>MGTFTLHQGQTNLIKSFFRNYYLNAELELPKDMELREFALQPFGSDTYVRHLSFSSSEELRDYLVNRNLPLHLFYSSARYQLPSARNMEEKAWMGSDLLFDIDADHLCKLRSIRFCPVCGNAVVSEKCERDNVETLEYVEMTSECIKRGLEQTRNLVEILEDDFGLKPKVYFSGNRGFHVQVDCYGNCALLDSDERKEIAEYVMGIGVPGYPGGSENAPGWVGRKNRGINGVTIDEQVTIDVKRLIRIPNSLHGKSGLIVKRVPNLDDFEFNETLSPFTGYTIFLPYITIETEVLGSIIKLNRGIPIKIKSSIGIYLHLRNLGEVKAYVR[2x];>MALDVKKYPFIKSLDDELKKYGGGITLTDLLLNSTTLIDQAKDRIQKTKSGDELPHYVSYNEPVLVFYTTLLSLAILNDVKLIRRYAYAEAKQFRSLLHTENEENLLEISKLLDLKINRCDPIKFYLEKKRRIIQKEFCVHFIDYLKYTKDLKEDWKLSGQILHKGYVYLDKNQLIGLIAESIKSKIVEMIRPLNLKEIPEKLKSLIERRGIIPPCIENILAKEKLNEEEIRTLITFYIDIGKGLSGIVSIMKKYNVSNVEDLYRKYRGDKGTRYIVYSCAKMKQLGLCVSSCNVKNPLQLYFLSNE[2x];>[2x]MSQEKKAKKIILHYPDDTPAGYIEYAEGSSSIYDNEGNFLFKVEGKFPPQPKKSSDYSWIEKVLEMGLQDSRKRFILYVASRYLVNVKGVNEDEALQTLKEFYYKLQSGKVYESWLKSVINGVKKKGLLPWSLKRIEERDKEMYNEIIRVLKNS

Initiation of DNA synthesis during DNA replication relies on a specialised DNA-dependent RNA polymerase, known as primase. In archaea and eukarya, primase is a constitutive heterodimer of a catalytic subunit, PriS or Pri1, and a regulatory subunit, PriL or Pri27. PriX is required for primase activity and the protein is encoded by a gene that is essential for viability. We have shown that PriX has replaced the Fe–S cluster domain of PriL as the primase module responsible for endowing primase with the ability to initiate nucleic acid synthesis.

To determine a structural basis for the role of PriX in priming DNA synthesis during DNA replication, we determined the X-ray crystal structure of heterotrimeric PriSLX from S. solfataricus at 2.9 Å resolution. The PriSLX structure reveals that the six-helix bundle of globular PriX is docked within the concave arch formed by PriS and PriL, and is coplanar with them. PriSLX was crystallized in the presence of RNA/DNA and the non-hydrolysable nucleotide analog AMPCPP. Although no RNA/DNA was detected in the density map, two AMPCPP molecules were clearly visible. The first AMPCPP was bound in the active site of PriS, in what is considered the elongation site of primase12. The 2′-hydroxyl group of the ribose in the bound AMPCPP makes two hydrogen bonds to the main-chain carbonyl and nitrogen moieties of PriS L245 and R247, respectively. Interestingly, the second AMPCPP located in the density map was bound to PriX, at the edge of the PriX-PriS interface. The ribose of protein-bound AMPCPP remains exposed to solvent, whereas the adenine base becomes sandwiched between PriX and PriS. The side chains of the basic 72-RKR-74 motif in PriX contact the triphosphate, with R72 and R74 buttressed by supporting interactions provided by Y103 and D140, respectively. Alanine mutation of D70, R72, R74 abolish or severely impair the initiation step of primer synthesis, but leave unaffected the ability of primase to extend an existing primer, indicating that the NTP-binding site in PriX represents the initiation site of primase.Dynamic protein O-GlcNAcylation is achieved by the interplay of two essential enzymes; O-GlcNAc transferase (OGT) and O-GlcNAcase (OGA). Furthermore, bioinformatic analysis has suggested that the C-terminal domain of hOGA can adopt a GCN5 family acetyltransferase (AT)-like fold. Strikingly, close inspection of the OgOGA genomic location reveals an open reading frame coding for a predicted AT immediately downstream of the OgOGA gene. Sequence alignment of this predicted AT from O. granulosus (OgpAT) with the hOGA-AT domain (hOGA-AT) shows good similarity (30% sequence identity).

Crystals of OgpAT in complex with AcCoA formed in space group P3221 with one molecule in the asymmetric unit and synchrotron diffraction data were collected to 1.8 Å resolution. The structure of OgpAT consists of mixed α/β-fold, composed of a central seven-stranded twisted β-sheet (topology 1234576) sandwiched between six α-helices (two packed on one side of the β-core and four on the other). Despite low sequence homology, the overall fold identifies OgpAT as a member of the GCN5-related N-AT (GNAT) superfamily. The thioester group of AcCoA is sandwiched between strands β4 and β5. The side chain of Asn175, which is conserved among the GNAT members, donates a hydrogen bond to the amide oxygen of the CoA pantothenate/cysteamine link, while the NH of the same amide forms a hydrogen bond with the side chain of Asp137. The acetyl group of AcCoA forms a hydrogen bond with the backbone nitrogen of Ile136. Analysis of the OgpAT active site and comparison with the ternary complex of Naa50p reveals that His135 is in a position to function in catalysis. As expected from the crystallographic complex, wild-type OgpAT binds AcCoA (Kd = 8.7 μM).

> MASEVVIRRATAADHGDLCRVCLLTGDSGRDASSREDDPTLLGMIYAVPYQVGAPDFAFVLEDAEGVCGYLLGAPDTLSFQHFLEKEWLPPLRAGLTDPGPDPAAWQGSDWARDAIHRPPALPPIDLAAYPAHGHIDLLPRAQGRGVGSRAMDHLEAALAAAGAPGMHLQVSPENPRALGFYEHRGFRELCRSEDEVVVGRRLLDE>[3x]MELFSSDSEFTKIDSEAKPASTLPAFGFAFNASAPQFASLFTPL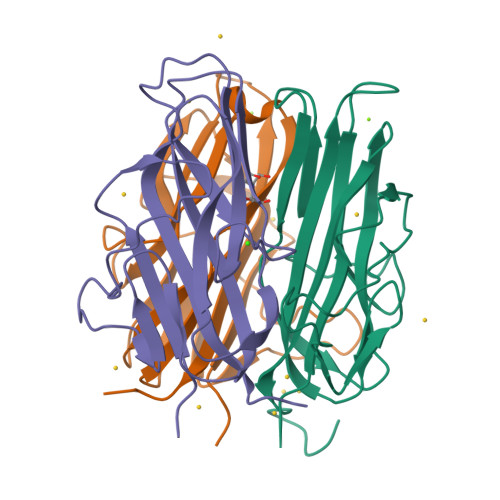LLPSVSPNPNITVPVINDTVSVGDGIRILRAGIYQISYTLTISLDNVPTAPEAGRFFLSLNTPANIIPGSGTAVRSNVIGTGEVDVSSGVILINLNPGDLIQIVPVELIGTVDIRAAALTVAQISRPHHHHHH> MHHHHHHASENLYFQGAMVMGNQQVVSITGAGSGIGLELVRSFKLAGYCVSALVRNEEQEALLCNEFKDALEIVVGDVRDHATNEKLIKQTIDRFGHLDCFIANAGIWDYMLNIEEPWEKISSSFDEIFDINVKSYFSGISAALPELKKTNGSVVMTASVSSHAVGGGGSCYIASKHAVLGMVKALAYELAPEIRVNAVSPGGTVTSLCGPASAGFDKMHMKDMPGIDDMIKGLTPLGFAAKPEDVVAPYLLLASRKQGKFITGTVISIDGGMA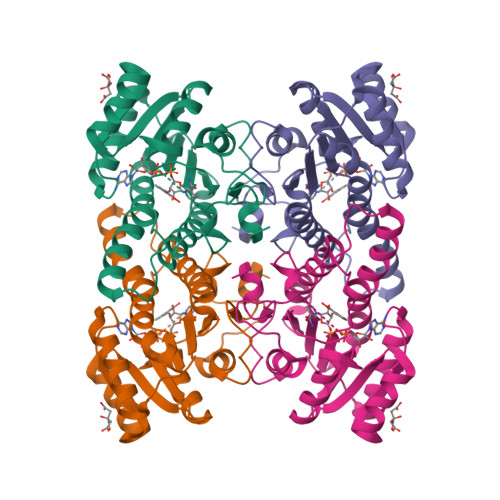LGRK>[4x]GIDPFTARPSSSMADFRKFFAKAKHIVIISGAGVSAESGVPTFRGAGGYWRKWQAQDLATPLAFAHNPSRVWEFYHYRREVMGSKEPNAGHRAIAECETRLGKQGRRVVVITQNIDELHRKAGTKNLLE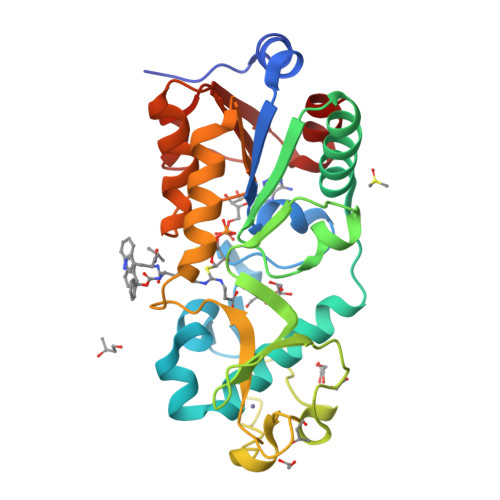IHGSLFKTRCTSCGVVAENYKSPICPALSGKGAPEPGTQDASIPVEKLPRCEEAGCGGLLRPHVVWFGENLDPAILEEVDRELAHCDLCLVVGTSSVVYPAAMFAPQVAARGVPVAEFNTETTPATNRFRFHFQGPCGTTLPEALA>[2x]M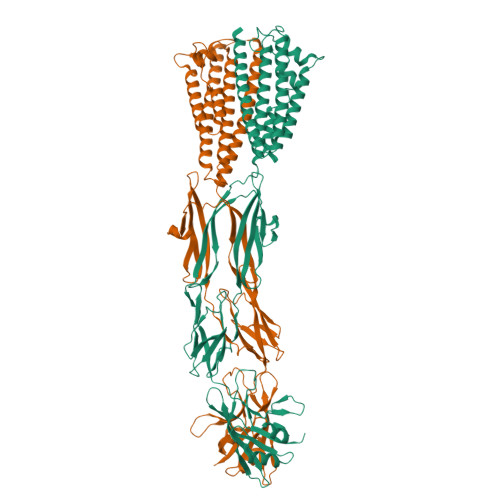DIGINSDPMAVGSNGNANRQKMINLMYLVFIAMMALNVSSEVLDGFDKVDKSLTSSIDGSDKRNNLVLSELNTAYRTNPEKVKVWYERSLVLQKEADSLCTFIDDLKLAIARESDGKDAKVNDIRRKDNLDASSVVMLNPINGKGSTLRKEVDKFRELVATLMTDKAKLKLIEQALNTESGTKGKSWESSLFENMPTVAAITLLTKLQSDVRYAQGEVLADLVKSVDVGDYRVNSITAQVIPQSQIVMSGDTYKANIVLSSVDTTQRPDVFVNGKLLSPENMGLFTATAGAPGTYPVKGYIEMMGNDGVKIRRDFESEYFVTEPMASVAPTMMNVLYAGIDNPINIAVPGVAQQNVSATINNGTLTRRGNLWIARPTKVGSEAIISVTAQSGGRTIQMAKTTLRVRALPDPLPYIEYKDVQGNTKRFKGGRLGKREILAAGGIKAALDDDLLEVNYTVVKFQLVFYDSMGNSIPEVSDGASFSERQKRQIQNLGKGKRFYVTEVIARGPDGIERKIPAIEVIVNLEHHHHHH(5R,10S)-5-{[(CARBOXYMETHYL)AMINO]CARBONYL}-7-OXO-3-THIA-1,6-DIAZABICYCLO[4.4.1]UNDECANE-10-CARBOXYLIC 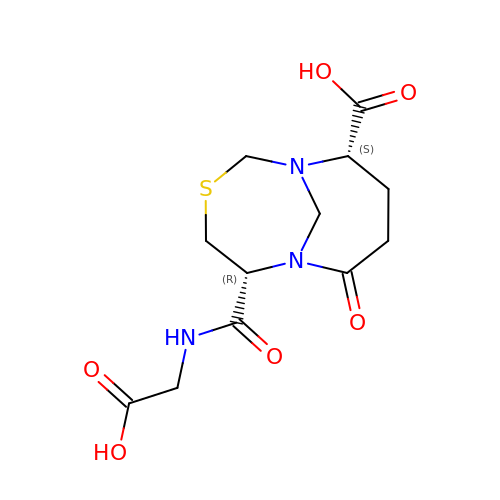ACID | C12 H17 N3 O6 S | FNEMNSFAPZMNDP-YUMQZZPRSA-N>MVRIAVAGAAGRMGRNLVKAAHHNPVAKVAAGSERPESSLVGVDLGELCGEGKFDVVVCDDLAKQIDQFDVIIDFTAPASTLNNLALCQQYGKSIVIGTTGFTEEQREQIDLVAQQVPVVMAPNYSVGVNLVFKLLEKAAKVMGDYCDIEIVEAHHRHKVDAPSGTAIGMGEAIAGAMGNKLSDVAVYAREGITGERTKDEIGFA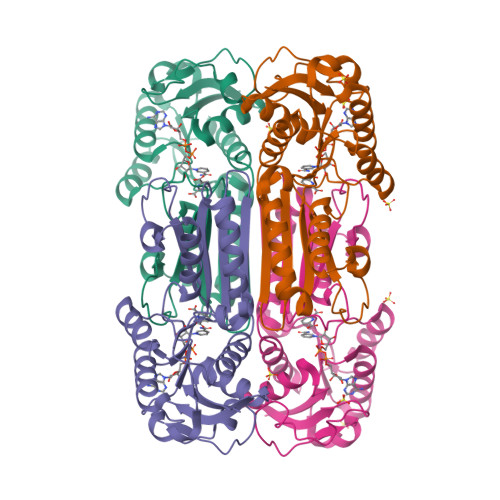TIRAGDIVGEHTAMFADIGERVEITHKATDRMTFANGAVKAAVWLHEKPAGFYTMTDVLGLNDL[2x]>[2x]TRQMILAVGQQGPIARAETREQVVVRLLDMLTKAA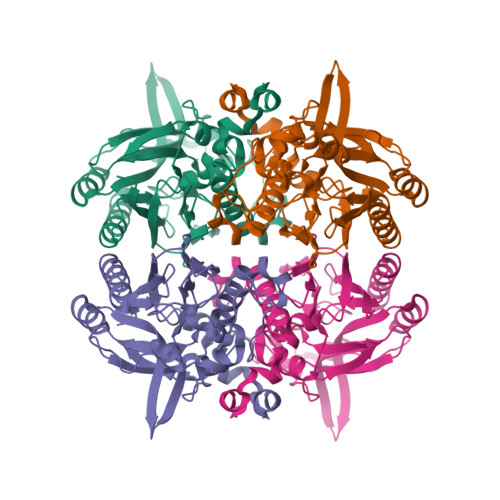SRGANFIVFPELALTTFFPRWHFTDEAELDSFYETEMPGPVVRPLFEKAAELGIGFNLGYAELVVEGGVKRRFNTSILVDKSGKIVGKYRKIHLPGHKEYEAYRPFQHLEKRYFEPGDLGFPVYDVDAAKMGMFIANDRRWPEAWRVMGLRGAEIICGGYNTPTHNPPVPQHDHLTSFHHLLSMQAGSYQNGAWSAAAGKAGMEENCMLLGHSCIVAPTGEIVALTTTLEDEVITAAVDLDRCRELREHIFNFKQHRQPQHYGLIAEL> MAVIAFGKFKLNLGTREMFREDEPMPLTSGEFAVLKALVSHPREPLSRDKLMNLARGREYSA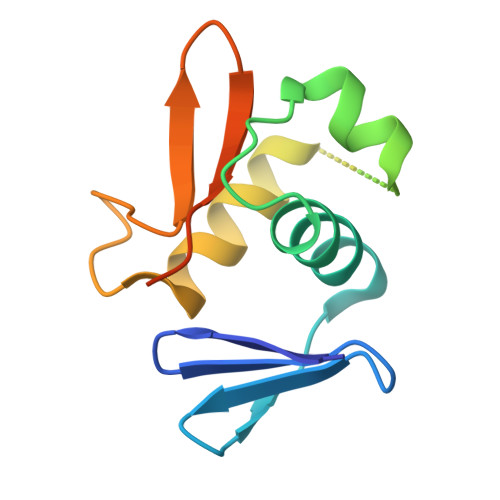MERSIDVQISRLRRMVEEDPAHPRYIQTVWGLGYVFVPDGSKALEHHHHHH>[2x]MAKGGSRVSNPAVMAQEEEDVRDYNLTEEQKAIKAKYPPVNRKYEYLDHTADVQLHAWGDTLEEAFEQCAMAMF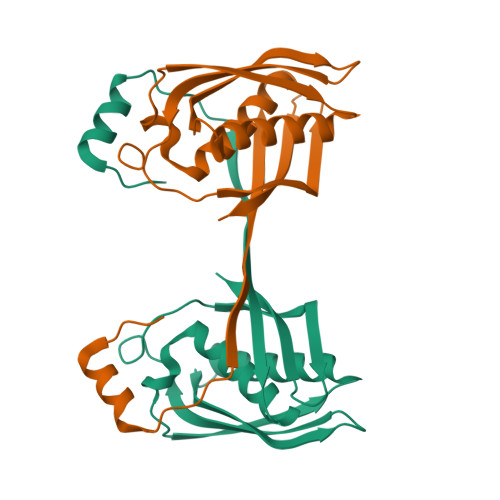GYMTDTGTVEPLQTVEVETQGDDLQSLLFHFLDEWLYKFSADEFFIPREVKVLSIDQRNFKLRSIGWGEEFSLSKHPQGTEVKAITYSAMQVYNEENPEVFVIIAILEHHHHHH> GG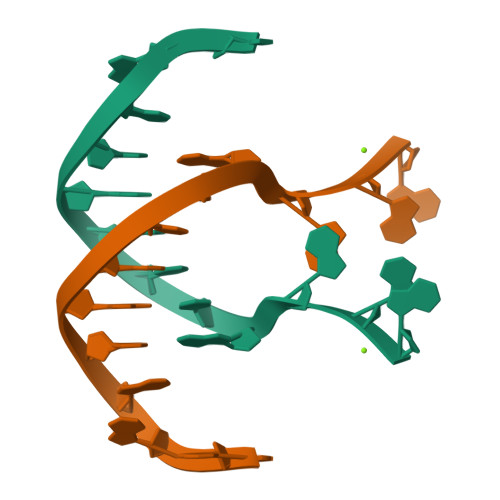AATCGATGGAG> MSEIILTPKEQPEVPLEAPNIKPDVFAGKSIEEIKNIQIMHGNEVVKLGDFFEVSGEPADAPEDI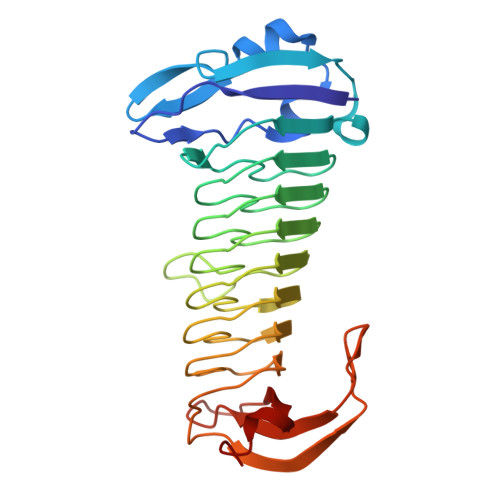KIIIDGDVYNTKRIGQEMTAGEIIVRGNVNMYVGAGMKGGKITVEGNAGSWAGQDMRGGEIEILGDAGDYVGSSYRGDWRGMSGGTITVHGNADNEIGEYMNGGKIIIKGDVNIMPGIHMNNGLIIIEGNVVARAGGEMAGGTIVVKGMMQEFLAGFKYLGVEKDIEVDGEELPGAFYKFEGDHAIKGAKGIVYAAVGCNGHIAP>MSLDSRLPAFRNLSPAARLDHIGQLLGLSHDDVSLLANAGALPMDIANGMIENVIGTFELPYAVASNFQINGRDVLVPLVVEEPSIVAAASYMAKLARANGGFTTSSSAPLMHAQVQIVGIQDPLNARLSLLRRKDEIIELANRKDQLLNSLGGGCRDIEVHTFADTPRGPMLVAHLIVDVRDAMGANTVNTMAEAVAPLMEAITGGQVRLRILSNLADLRLARAQVRITPQQLETAEFSGEAVIEGILDAYAFAAVDPYRAATHNKGIMNGIDPLIVATGNDWRAVEAGAHAYACRSGHYGSLTTWEKDNNGHLVGTLEMPMPVGLVGGATKTHPLAQLSLRILGVK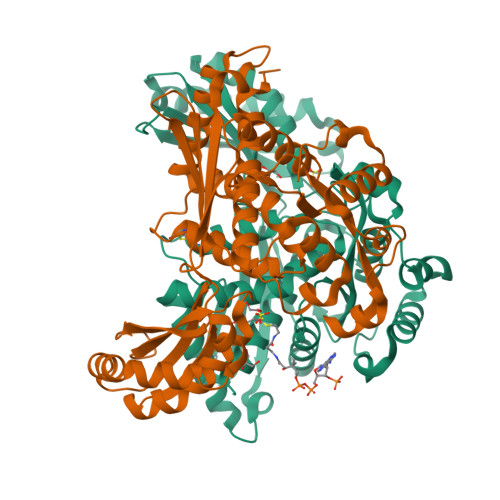TAQALAEIAVAVGLAQNLGAMRALATEGIQRGHMALHARNIAVVAGARGDEVDWVARQLVEYHDVRADRAVALLKQKRGQ[2x]>EVSQDLFNQFNLFAQYSAAAYCGKNNDAPAGTNITCTGNACPEVEKADATFLYSFEDSGVGDVTGFLALDNTNKLIVLSFRGSRSIENWIGNLNFDLKEINDICSGCRGHDGFTSSWRSVADTLRQKVEDA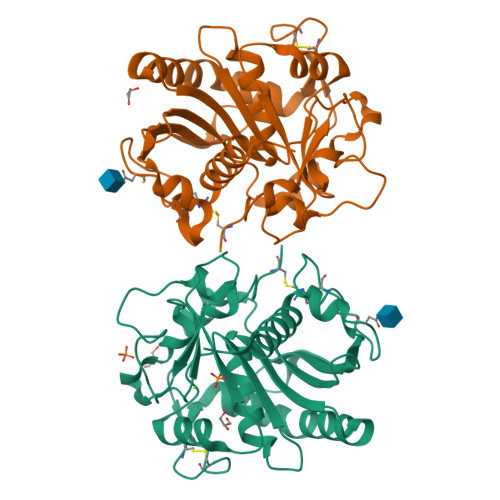VREHPDYRVVFTGHSLGGALATVAGADLRGNGYDIDVFSYGAPRVGNRAFAEFLTVQTGGTLYRITHTNDIVPRLPPREFGYSHSSPEYWIKSGTLVPVTRNDIVKIEGIDATGGNNQPNIPDIPAHLWYFGLIGTCL[2x]> NEQSGISQTVIVGPWGAQ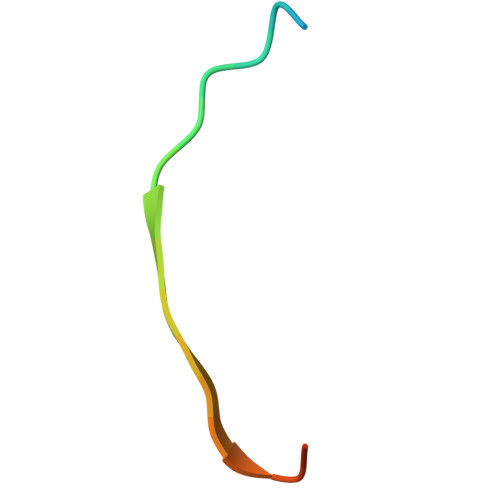VST> SQAAADRRTVEKTWKLMDKVVRLCQNPKLQLKNSPPYILDILPDTYQHLRLILSKYDDNQKLAQLSENEYFKIYIDSLMKKSKRAIRLFKEGKERMYEEQSQDRRNLTKLSLIFSHMLAEIKAIFPNGQFQGDNFRITKADAAEFWRKFFGDKTIVPWKVFRQ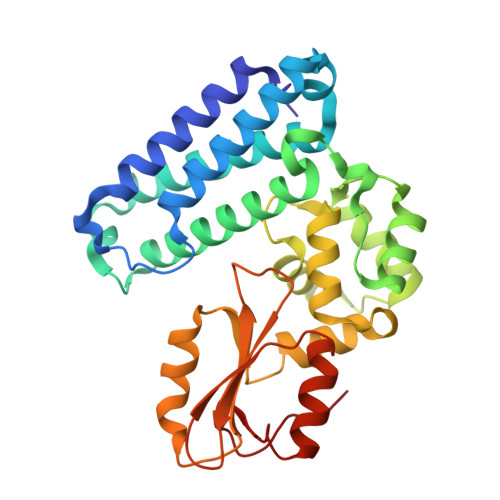CLHEVHQISSGLEAMALKSTIDLTCNDYISVFEFDIFTRLFQPWGSILRNWNFLAVTHPGYMAFLTYDEVKARLQKYSTKPGSYIFRLSCTRLGQWAIGYVTGDGNILQTIPHNKPLFQALIDGSREGFYLYPDGRSYNPDLTG>[6x]MNHKVHHHHHHMGGGSTPLPLPQQQPPQQEPPPPPVPLASRAACEALKDGNGDMVWPNAATVVEVAAWRDAAPATA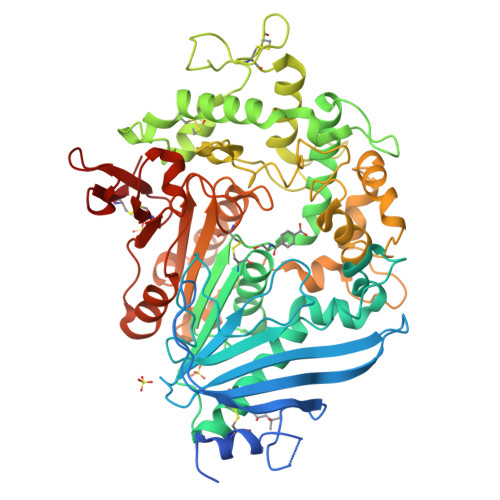SAAALPEHCEVSGAIAKRTGIDGYPYEIKFRLRMPAEWNGRFFMEGGSGTNGSLSAATGSIGGGQIASALSRNFATIATDGGHDNAVNDNPDALGTVAFGLDPQARLDMGYNSYDQVTQAGKAAVARFYGRAADKSYFIGCSEGGREGMMLSQRFPSHYDGIVAGAPGYQLPKAGISGAWTTQSLAPAAVGLDAQGVPLINKSFSDADLHLLSQAILGTCDALDGLADGIVDNYRACQAAFDPATAANPANGQALQCVGAKTADCLSPVQVTAIKRAMAGPVNSAGTPLYNRWAWDAGMSGLSGTTYNQGWRSWWLGSFNSSANNAQRVSGFSARSWLVDFATPPEPMPMTQVAARMMKFDFDIDPLKIWATSGQFTQSSMDWHGATSTDLAAFRDRGGKMILYHGMSDAAFSALDTADYYERLGAAMPGAAGFARLFLVPGMNHCSGGPGTDRFDMLTPLVAWVERGEAPDQISAWSGTPGYFGVAARTRPLCPYPQIARYKGSGDINTEANFACAAPP N-(2-(2-cyclopropylethoxy)pyrimidin-5-yl)-7-methoxy-6-(piperidin-4-ylmethoxy)quinazolin-4-amine 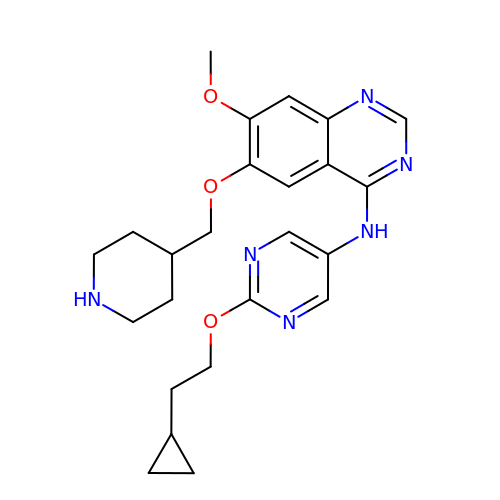| C24 H30 N6 O3 | PLIIPGVTCVYGIU-UHFFFAOYSA-N>GSHMSQSLFSLAFGVGTQNRQEAWLEVFYALPLLKPSSEIVAAVAPILGYAAGNQALTFTSQQAYQLADALKGIDAAQSALLSRLAESQKPLVATLLAEDAAPSSTAEAYLKLHLLSHRLVKPHAVNLSGIFPLLPNVAWTNIGAVDLAELAELQLEARLKGKLLEVFSVDKFPKMTDYVVPAGVRIADTARVRLGAYIGEGTTVMHEGFVNFNAGTEGPGMIEGRVSAGVFVGKGSDLGGGCSTMGTLSGGGNIVISVGEGCLIGANAGIGIPLG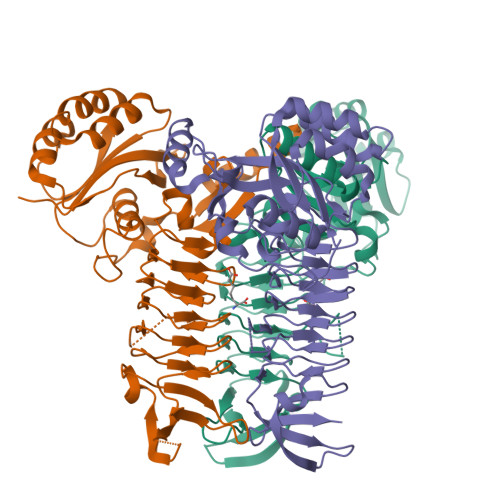DRNIVEAGLYITAGTKVALLDEQNALVKVVKARDLAGQPDLLFRRNSQNGAVECKTNKTAIELNEALHAHN[6x]> MKIIILGAGQVGGTLAENLVGENNDITIVDNNADRLRELQDKYDLRVVNGHASHPDVLHEAGAQDADMLVAVTNTDETNMAACQVAFTLFNTPNRVARIRSPEYLAEKEALFKSGAIPVDHLIAPEELVTSYIERLIQYPGALQVVSFAEQKVSLVAVKAYYGGPLVGNALSALREHMPHIDTRVAAIFRQGRPIRPQGTTIIEADDEVFFVAASNHIRSVMSELQRLEKPYRRIMIVGGGNIGASLAKRLEQTYSVKLIERDYQRAEKLSEQLENTIVFCGDAADQELLTEENIDQVDVFIALTNEDETNIMSAMLAKRMGAKKVMVLIQRGAYVDLVQGGVIDVAISPQQATISALLTHVRRADIVNVSSLRRGAAEAIEAVAHGDETTSKVVGRAIGDIKL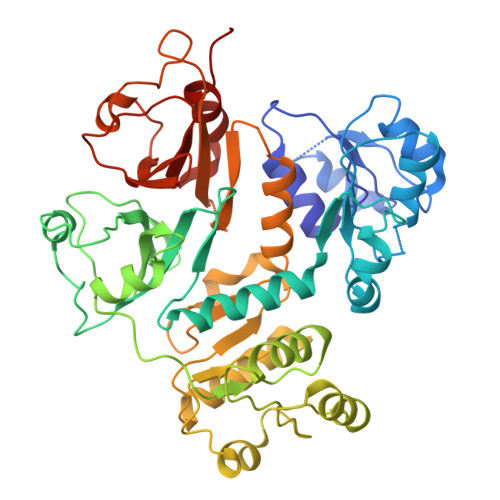PPGTTIGAVVRGEEVLIAHDRTVIEQDDHVVMFLVDKKYVPDVEALFQPSPFFL>[4x]SKDAPQSKFFQPVLKPMLPPDAFQGKVAFITGGGT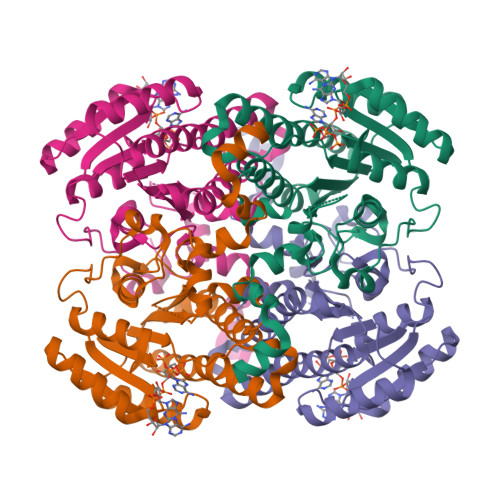GLGKAMTTFLSTLGAQCVIASRNIDVLKATAEEISSKTGNKVHAIRCDVRDPDMVHNTVLELIKVAGHPDVVINNAAGNFISPSERLTPNGWKTITDIVLNGTAYVTLEIGKQLIKAQKGAAFLAITTIYAESGSGFVMPSSSAKSGVEAMNKSLAAEWGRYGMRFNIIQPGPIKTKGAFSRLDPTGRFEKEMIDRIPCGRLGTMEELANLATFLCSDYASWINGAVIRFDGGEEVFLSGEFNSLKKVTKEEWDIIEGLIRKTKGS>GPLGSDGGRFKGDLPEERHMKVDNKNFYFDIGQNNRGVYMRISEVKNNFRTSITIPEKCWIRF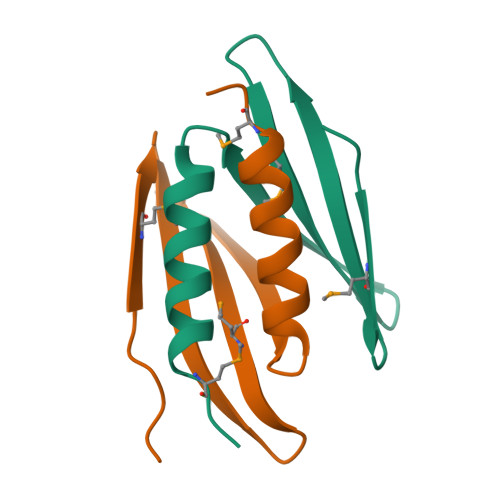RDIFNDYCEKMKKSSDSI[6x]(1-AMINO-PENTYL)-PHOSPHONIC 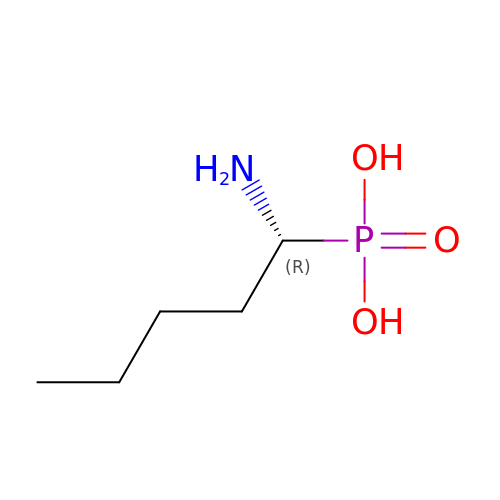ACID | C5 H14 N O3 P | NXTPDFMZKSLVRK-RXMQYKEDSA-N> MNQTLETGTTTVGITLKDAVIMATERRVTMENFIMHKNGKKLFQIDTYTGMTIAGLVGDAQVLVRYMKAELELYRLQRRVNMPIEAVATLLSNMLNQVKYMPYMVQLLVGGIDTAPHVFSIDAAGGSVEDIYAS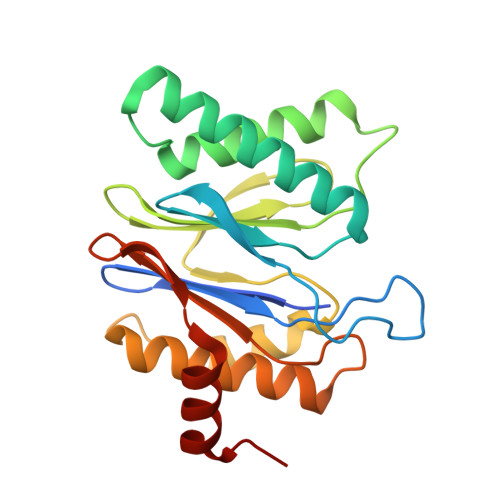TGSGSPFVYGVLESQYSEKMTVDEGVDLVIRAISAAKQRDSASGGMIDVAVITRKDGYVQLPTDQIESRIRKLGLIL(2R,5S,10R)-6,10-dimethyl-2-(prop-1-en-2-yl)spiro[4.5]dec-6-ene | C15 H24 | 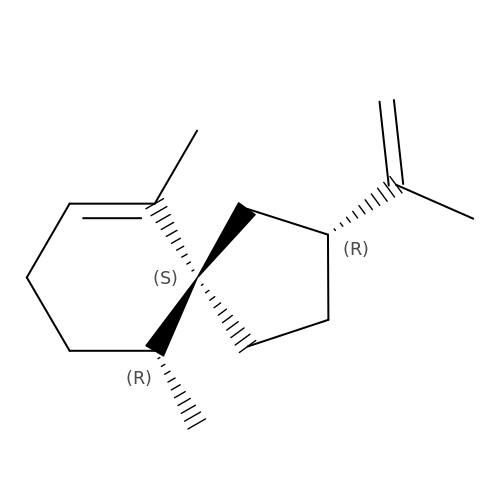WEZDOYDDKIHCLM-RBSFLKMASA-N> MQHYLHIRPAPSDNLPLVDLIEHPDPIFDPKEKDLNETLLRSLLGGHYDPGFMATSPPEDRPGGGGGAAGGAEDLAELDQLLRQRPSGAMPSEIKGLEFSEGLAQGKKQRLSKKLRRKLQMWLWSQTFCPVL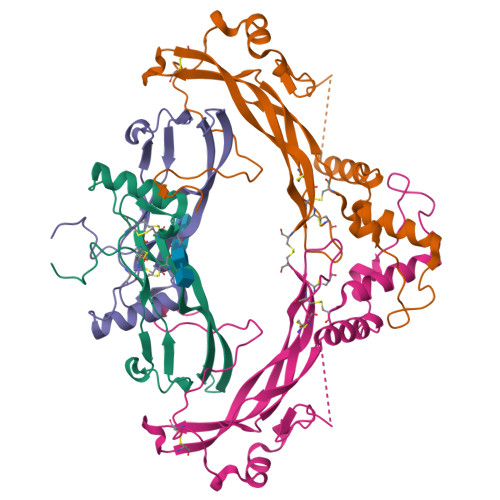YAWNDLGSRFWPRYVKVGSCFSKRSCSVPEGMVCKPSKSVHLTVLRWRCQRRGGQRCGWIPIQYPIISECKCSC;> STGSKQRSQNRSKTPKNQEALRMANVAENSSSDQRQACKKHELYVSFRDLGWQDWIIAPEGYAAYYCEGECAFPLNSYMNATNHAIVQTLVHFINPETVPKPCCAPTQLNAISVLYFDDSSNVILKKYRNMVVRACGCH> TTSGWVKQDGAWYYFDGNGNLVKNAWQGSYYLKADGKMAQSEWIYDSSYQAWYYLKSDGSYAKNAWQGAYYLKSNGKMAQGEWVYDSSYQAWYYLKSDGSYARNAWQGNYYLKSDGKMAKGEWVYDATYQAWYYLTSDGSYAYSTWQGNYYLKSDGKMAVNEWVDGGRYY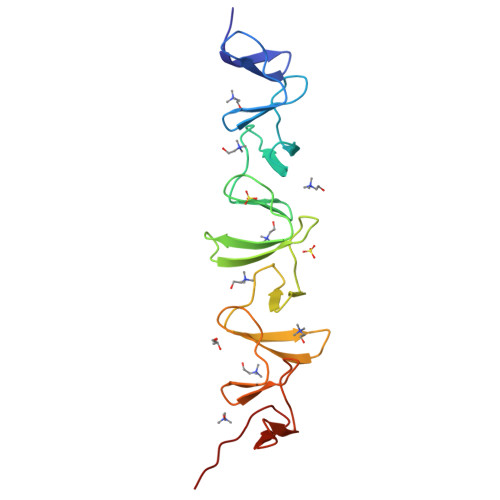VGADGVWKEVQA SET domain methyltransferases deposit methyl marks on specific histone tail lysine residues and play a major role in epigenetic regulation of gene transcription. HKMTs catalyze the transfer of a methyl group from the co-factor S-adenosyl-L-methionine (SAM) to a substrate lysine and, with the exception of DOT1L, are all organized around a canonical SET domain. Methylation of H3K9 in humans relies mostly on members of the Suv39 family, namely EHMT1/GLP, EHMT2/G9a, SUV39H1, SUV39H2, SETDB1 and SETDB2, as well as then non-Suv39 enzymes PRDM2 and ASH1L. Here we report the high-resolution crystal structures of the methyltransferase domains of GLP, G9a, SUV39H2 and PRDM2, and propose a structural mechanism for substrate recognition.

The specificity of PRDM2 is unknown. Unlike I-SET, Post-SET is absent from the PRDM2 structure, which lacks co-crystallized SAM or SAH. The Post-SET domains of G9a, GLP, SUV39H2, but not PRDM2 include a ZnCys motif previously observed in the structures of Dim-5 and the H3K4 methyltransferase MLL1. (1) A flexible or even disordered state when no co-factor or peptide is bound. Mapping the electrostatic potential along the molecular surface of GLP, G9a, SUV39H2 and PRDM2 shows that the peptide-binding groove is consistently electronegative.

> GSNQNTTEPVAATETLAEVPEHVLRGLPEEVRLFPSAVDKTRIGVWATKPILKGKKFGPFVGDKKKRSQVKNNVYMWEVYYPNLGWMCIDATDPEKGNWLRYVNWACSGEEQNLFPLEINRAIYYKTLKPIAPGEELLVWYNGEDNPEI>MRKLKYNTTRVILMIAFISLSACSSEDAMIEEEQVIPDPDPVAQTDEDTGPVVDCTNQGTNPTRDTDIPNPRNIGDIDDRSCYANYSESSILGKFWGIYNITDGSNHMDAPNTLQPRIERSLSRSQATGAGSYARFRGVLRILEVGDTGTFSSSGSYFMQAMGKHTGGGGSPDPAICLYRAHPVYGDDGNGNQVQVSFDIWREQINFRGGSGSAGRTEVFLKNVLKNEQIDIELEVGFRDDPNNPGQTLHYADAKIGGEEFNWNIPEPERGIESGIRYGAYRVKGGRAQFRWANTSYTKDEV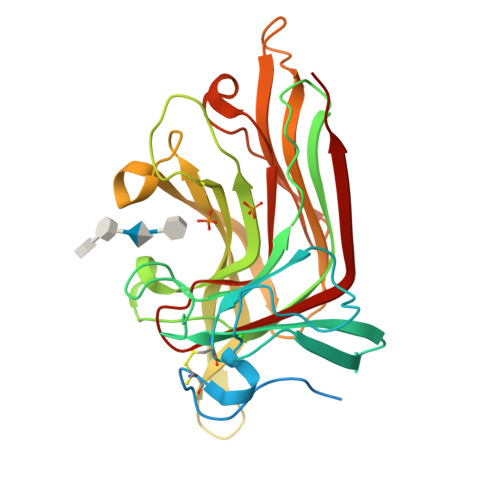N[2x]>[2x]TQKPSLYRVLILNDDYTPMEFVVYVLERFFNKSREDATRIMLHVHQNGV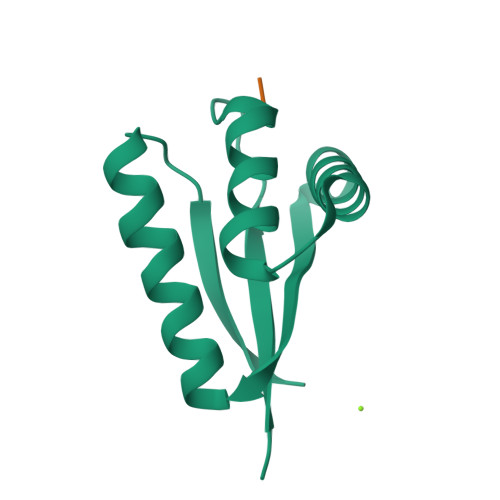GVCGVYTYEVAETKVAQVIDSARRHQHPLQCTMEKD;>[2x]FGG> MAGAIENARKEIKRISLEDHAESEYGAIYSVSGPVVIAENMIGCAMYELVKVGHDNLVGEVIRIDGDKATIQVYEETAGLTVGDPVLRTGKPLSVELGPGLMETIYDGIQRPLKAIKEESQSIYIPRGIDTPALDRTIKWQFTPGKFQVGDHISGGDIYGSVFENSL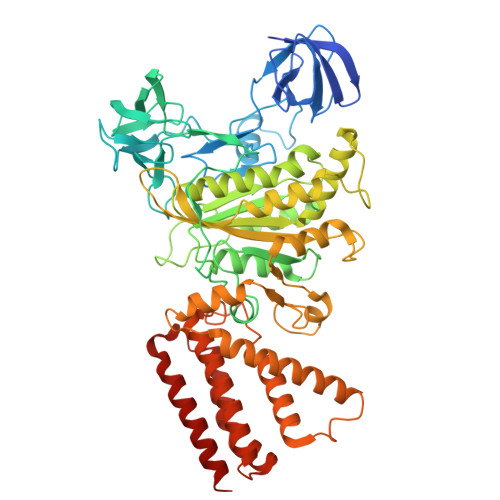ISSHKILLPPRSRGTITWIAPAGEYTLDEKILEVEFDGKKSDFTLYHTWPVRVPRPVTEKLSADYPLLTGQRVLDALFPCVQGGTTCIPGAFGCGKTVISQSLSKYSNSDAIIYVGCGERGNEMAEVLMEFPELYTEMSGTKEPIMKRTTLVANTSNMPVAAREASIYTGITLAEYFRDQGKNVSMIADSSSRWAEALREISGRLGEMPADQGFPAYLGAKLASFYERAGKAVALGSPDRTGSVSIVAAVSPAGGDFSDPVTTATLGITQVFWGLDKKLAQRKHFPSINTSVSYSKYTNVLNKFYDSNYPEFPVLRDRMKEILSNAEELEQVVQLVGKSALSDSDKITLDVATLIKEDFLQQNGYSTYDAFCPIWKTFDMMRAFISYHDEAQKAVANGANWSKLADSTGDVKHAVSSSKFFEPSRGEKEVHGEFEKLLSTMQERFAESTD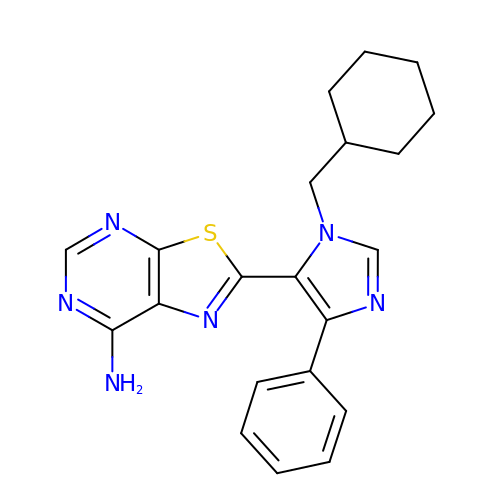2-[3-(CYCLOHEXYLMETHYL)-5-PHENYL-IMIDAZOL-4-YL]-[1,3]THIAZOLO[4,5-E]PYRIMIDIN-7-AMINE | C21 H22 N6 S | FACMGTJQTMTYEF-UHFFFAOYSA-N>MGGSEYRVDLVVLSEQKQNCRFGLTFHNLSDQDLNSWGLTFAFDRYILPDSVSNGQLTQIGSFCTLKPEGIVLAANHHYYCEFSIGSNPFRYYSDGFNEAMIDFVVDGQPQRAQVDVTPIVLASPYRERSDIPASLTHAQPLLPKPNHIEVSDHSFTFDEQAGVAIYTDLANSAKAWLLEELQRIHQFTLSSSNSGKIIFKSNPTLDEGAYKLKVSEESIKIEAGSSSGFTHACATLLQLLKRDEATKTMEAVCCSIIDSPRFRYRGMMLDCARHFHSVEQVKRLINLLAHYKLNTFHWHLTDDEGWRVEIKSLPQLTEIGAWRGIDETIEPQYTHLSQRYGGFYTQEEIRDVIAFAEQRGITIIPEIDVP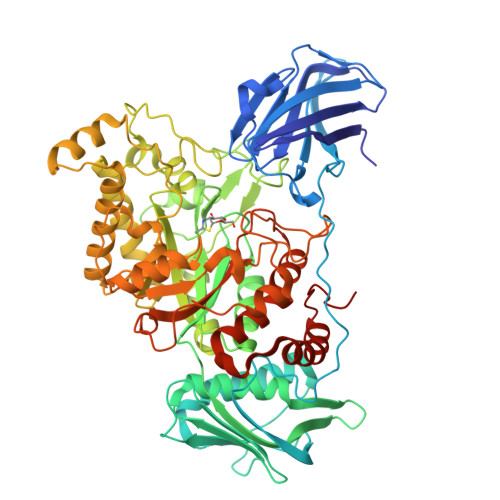GHCRAAIKSLPHLLIEAEDTTEYRSIQHYNDNVINPALPGSYEFIDKVLEEIAALFPAPYVHIGADEVPNGVWSKSPACQALMEQLGYTDYKELQGHFLRHAEDKLRKLGKRMLGWEEAQHGNKVSKDTVIYSWLSEEAALNCARQGFDVVLQPAQTTYLDMTQDYAPEEPGVDWANPLPLEKAYNYEPLAEVPADDPIRKRIWGIQTALWCEIINNPSRMDYMIFPRLTAMAEACWTEKQHRDWTDYLSRLKGHLPLLDLQGVNYRKPWKRSRSHHHHHH[2x]>MYQDLIRSELTEAADVLQKFLSDDHNIAQIEAAAKLIADSFKQGGKVLSCGNGGSHCDAMHFAEELTGRYRENRPGYPGIAISDPSHLSCVSNDFGYDYVFSRYVEAVGAKGDVLFGLSTSGNSGNILKAIEAAKAKGMKTIALTGKDGGKMAGLADVEIRVP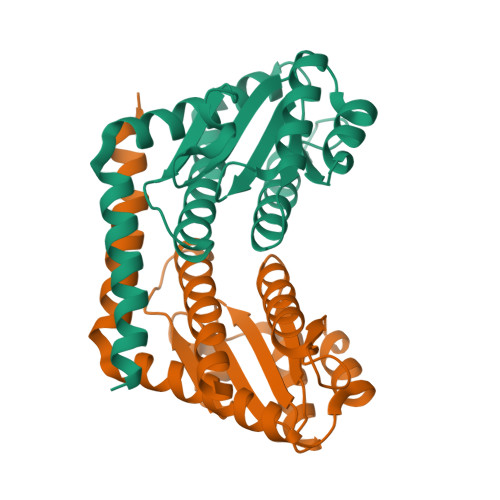HFGYADRIQEVHIKIIHIIIQLIEKEMA[2x]> IVQDVPNAPKLTGITCQADKAEIHWEQQGDNRSPI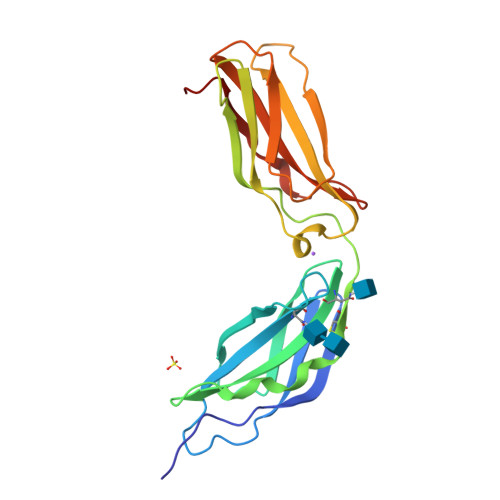LHYTIQFNTSFTPASWDAAYEKVPNTDSSFVVQMSPWANYTFRVIAFNKIGASPPSAHSDSCTTQPDVPFKNPDNVVGQGTEPNNLVISWTPMPEIEHNAPNFHYYVSWKRDIPAAAWENNNIFDWRQNNIVIADQPTFVKYLIKVVAINDRGESNVAAEEVVGYSGEDR> AHRKPSLLA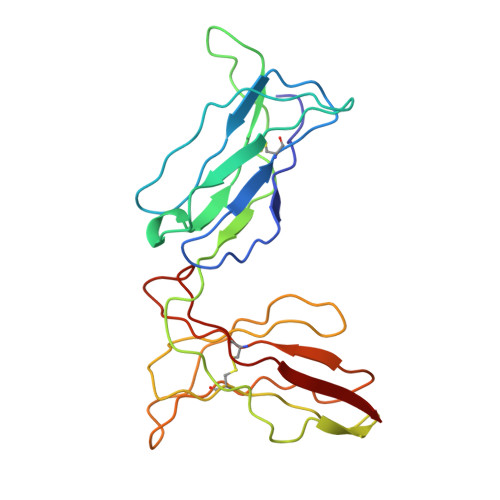HPGRLVKSEETVILQCWSDVRFEHFLLHREGKFKDTLHLIGEHHDGVSKANFSIGPMMQDLAGTYRCYGSVTHSPYQLSAPSDPLDIVITGLYEKPSLSAQPGPTVLAGESVTLSCSSRSSYDMYHLSREGEAHECRFSAGPKVNGTFQADFPLGPATHGGTYRCFGSFRDSPYEWSNSSDPLLVSVI> MGMSKSHSFFGYPLSIFFIVVNEFCERFSYYGMRAILILYFTNFISWDDNLSTAIYHTFVALCYLTPILGALIADSWLGKFKTIVSLSIVYTIGQAVTSVSSINDLTDHNHDGTPDSLPVHVVLSLIGLALIALGTGGIKPCVSAFGGDQFEEGQEKQRNRFFSIFYLAINAGSLLSTIITPMLRVQQCGIHSKQACYPLAFGVPAALMAVALIVFVLGSGMYKKFKPQGNIMGKVAKCIGFAIKNRFRHRSKAFPKREHWLDWAKEKYDERLISQIKMVTRVMFLYIPLPMFWALFDQQGSRWTLQATTMSGKIGALEIQPDQMQTVNAILIVIMVPIFDAVLYPLIAKCGFNFTSLKKMAVG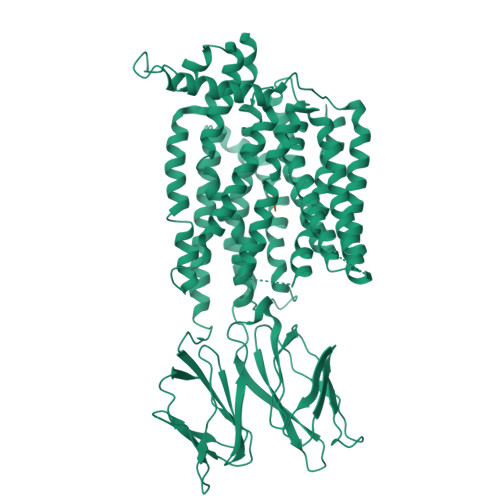MVLASMAFVVAAIVQVEIDKTLPVFPKGNEVQIKVLNIGNNTMNISLPGEMVTLGPMSQTNAFMTFDVNKLTRINISSPGSPVTAVTDDFKQGQRHTLLVWAPNHYQVVKDGLNQKPEKGENGIRFVNTFNELITITMSGKVYANISSYNASTYQFFPSGIKGFTISSTEIPPQCQPNFNTFYLEFGSAYTYIVQRKNDSCPEVKVFEDISANTVNMALQIPQYFLLTCGEVVFSVTGLEFSYSQAPSNMKSVLQAGWLLTVAVGNIIVLIVAGAGQFSKQWAEYILFAALLLVVCVIFAIMARFYTYINPAEIEAQFDEDEKKNRLEKSNPYFMSGANSQKQM;> AF> GGGHMAKIIVKKSNPLKGSVKIDGAKNAVLPIIAATLLANGKSTLNGVPNLRDVHVISDLLRHVGAEVEYKENTLTVDASNIKTCEAPYELVRKMRASFLVMGPLLARFNSTKISMPGGDAIGTRPIDLHLKGFKALGAKIEMDHGFVEAATEKLVGNKLYLDFPSVGATENIMMAASLAEGTTIIENAAEEPEIVDLANFLNEMGADVKGAGTNTIKIKGVKELKGAEHNVIPDRIEAATYMVAAAMTKGDITVENVLMEHL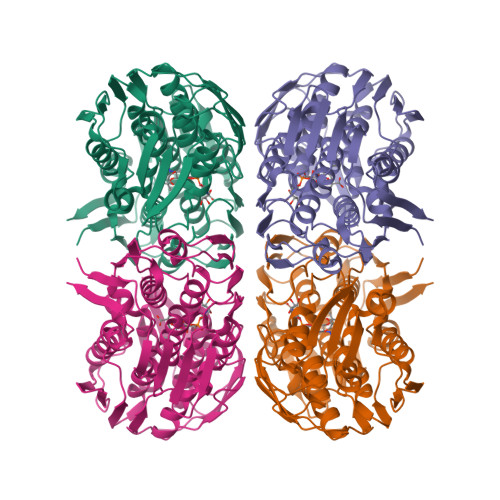KPVVAKLREAGCEITEMDNSVRVVGPKVLKPIDIKTLPHPGFPTDVQAQFMAMLTVANGTGVVIETVFENRFMHVAEFNRMGANIKIDGRSAVVNGVDELHGAAVNATDLRAGAALILCGLIAEGETQIGEIYHIQRGYVDIDKKITALGGQIEIVED One example is the fibrils formed from SAA1.1, the fibril precursor protein in systemic AA amyloidosis. Amyloid fibrils are fibrillar polypeptide aggregates which occur in a range of diseases that includes several neurodegenerative diseases and different forms of systemic amyloidosis. The fibrils can have a length of serval micrometers and consist of cross-β structure and of β-strands that run roughly perpendicular to the fibril main axis. In this research we use cryo-electron microscopy and other methods to analyze the ability of serum amyloid A (SAA).1-derived amyloid fibrils, purified from systemic AA amyloidosis tissue, to seed solutions of recombinant SAA1.1 protein.

To clarify its molecular assembly, we obtained the cryo-EM structure of the major seeded in vitro fibril morphology at a resolution of 2.69 Å, based on 0.143 Fourier shell correlation (FSC) criterion. The fibril contains two protofilaments that are arranged with a pseudo 21 screw symmetry. These properties resemble the previously described ex vivo fibril morphology I. The helical parameters (rise 2.4 Å, twist 179.425°) of the seeded fibril are also very similar to the ex vivo fibril morphology (rise 2.41 Å, twist 179.44°). The stable structure of the fibril protein extends from Gly1 to Gly69. More C-terminal residues were not seen in the three-dimensional (3D) map, indicating structural disorder. The fibril protein fold of the seeded in vitro fibril corresponds to the fibril protein fold of ex vivo fibrils. The all atom root mean square deviation (RMSD) is 0.81 Å for the two fibril structures. The greatest similarity occurs at residues 51–64 (RMSD 0.46 Å), while the remaining part of the structures possesses an RMSD of 1.17 Å. Therefore, the greatest correspondence occurs at an inner radial position, where the two protofilaments are held together by reciprocal salt bridges between residues D59 and R61. Seeded in vitro fibrils were also stable to proteolytic digestion and persisted for more than 2 h under the conditions of our experiment, similar to the ex vivo fibrils.

>[12x]GFFSFIGEAFQGAGDMWRAYTDMKEAGWKDGDKYFHARGNYDAAQRGPGGVWAAEKISDARESFQEFFGRGHEDTMADQEANRHGRSGKDPNYYRPPGLPAKY VhCBP is a periplasmic chitooligosaccharide-binding protein mainly responsible for translocation of the chitooligosaccharide (GlcNAc)2 across the double membranes of marine bacteria. The chitooligosaccharide-specific SBP is localized to the periplasmic compartment of the bacterial cell wall and serves as a mobile component of the (GlcNAc)2-specific ABC transporter. SBPs share a common structural feature comprising two domains connected by a flexible hinge region. VcCBP and VhCBP belong to cluster C/subcluster IV (C-IV), members of which are specific for oligosaccharides, including mannooligosaccharides, cellooligosaccharides, and chitooligosaccharides.

Compared with the WT VhCBP, W363A not only eliminated the CH-π stacking interaction with the nonreducing end GlcNAc but also slightly shifted the Trp513 side chain and the bound (GlcNAc)2. These shifts may have altered the interaction of GlcNAc with amino acid side chains from the upper domain, including Trp513. As demonstrated from the crystal structure of W363A, the Trp513 side chain is shifted by the mutation of Trp363 by 0.6 Å, and the bound (GlcNAc)2 also shifted slightly. These rearrangements probably affect the binding interactions provided by amino acids in the upper domain, including Glu10, Asn204, Ser221, and Trp513. The mutational effects of Trp363 and Trp513 on ΔG° were similar (ΔΔG° = +4.7 ± 0.4 and +4.2 ± 0.3 kcal mol−1, respectively), but the effects of mutations on enthalpy/entropy contributions are significantly different between the two Trp mutants. The W363A mutation had a large effect on the enthalpic term, while in W513A, a large change was observed in the entropic contribution. Trp363 interacts purely through CH-π stacking, while Trp513 interacts through both CH-π stacking and hydrogen bonding with the N-acetyl group of the GlcNAc in site 1. Mutation of three conserved residues (Trp363, Asp365, and Trp513) to Ala resulted in drastic decreases in the binding affinity toward the preferred substrate (GlcNAc)2, indicating their significant contributions to sugar binding.

> AERSELTIHPKEFTTFVRNFNPFLGATNLHTTTDFIYEPLVVFNEMHGNTPVFRLAENFQMSDDLMSVTFDIRKGVKWSDGEAFTADDVVYSFNLVKEKPELDQSGINSWVTGVEKVNDYQVKFRLSEANSNVPYEIAKVPVVPKHVWSKVKDPSTFTNENPVGSGPFTVIDTFTPQLYIQCENPNYWDAANLDVDCLRVPQIANNDQFLGKVVNGEMDWTSSFVPDIDRTYAAASPKHHYWYPPAGTQAFVVNFKNPDAAKNEALTNVDFRRAFSMALDRQTIIDIAFYGGGTVNDFASGLGYAFEAWSDEKTHDKFKAYNSYNAEGAKKLLAKAGFKDVNKDGFVDTPSGKSFELLIQSPNGATDFNNTVQLAVEQLAEVGIKARARTPDFSVYNQAMLEGTYDVAYTNYFHGADPYTYWNSAYNSALQSGDGMPRFAMHFYKNEKLDGLLNSFYKTADKQEQLEIAHGIQQIIAQDQVTIPVLSGAYMYQYNTTRFTGWWNEENPKGRPNIWAGIPERLLHVLDLKPVKLEHHHHHH5-HYDROXY-3-OXOPENTANOIC ACID | C5 H8 O4 | 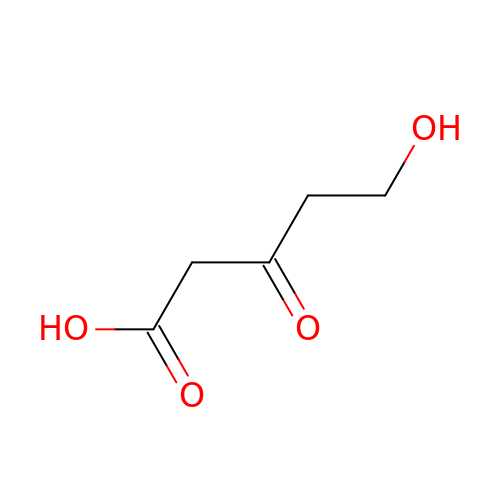ANTBRXMMNBUYMS-UHFFFAOYSA-N> 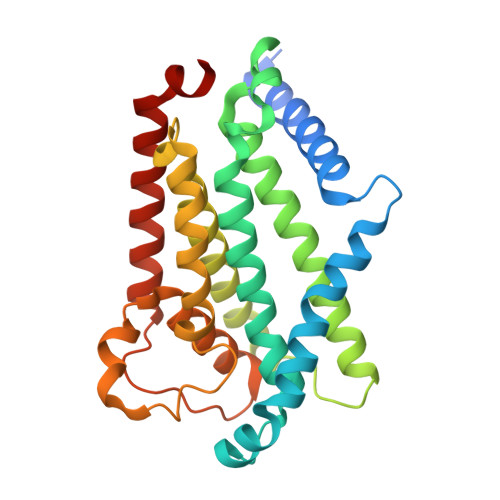MGKIHLAVSERSPRVKRSPWQIQQAVLFALFLRELKTRLGGRWLGVFWVLLEPVAHIAVMTTLFSLAHRAAMPSIEYPVFLITGLIPFFMFRGLVTRLMEAIDSNRGLFAYRQVKPIDTVIARAMLEISLQSIVYLIALGTLGWLGFHFLPVRALELAGVSAVLIMLGASLGLFFAVVTNEIPQARAIVRISLLPLYFVSGVIFPVHTIPPQYLPLLQLNPVLHLIELSRASFFPQYRVLQGINLAYPAGFALLSLFLALMLYRLRRHQLASVV>DHPFTEIKSGFLERRSKFLKSYSKGYYVLTPNFLHEFKTADRKKDLVPVMSLALSECTVTEHSRKNSTSSPNSTGSDAKFVLHAKQNGIIR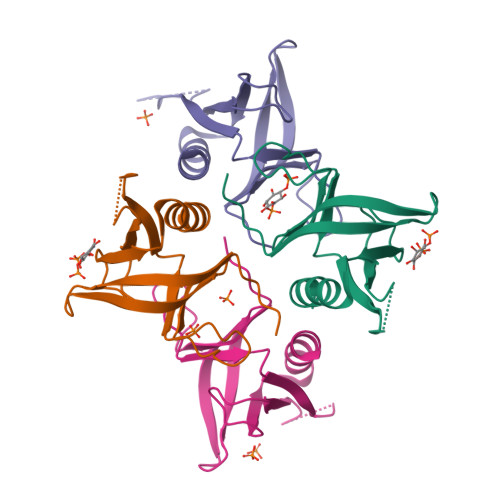RGHNWVFKADSYESMMSWFDNLKILTSTS[4x]> DQHFRGDNEEQEKLLKKSCTLY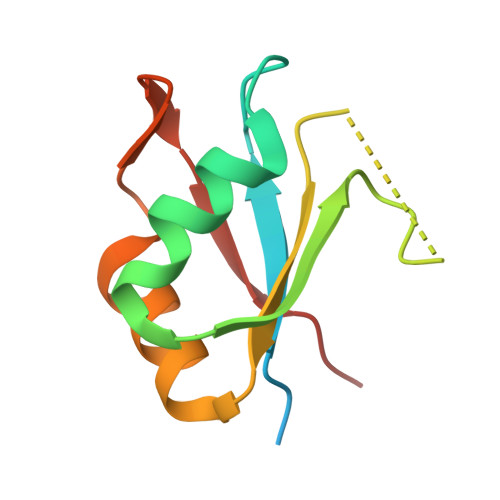VGNLSFYTTEEQIYELFSKSGDIKKIIMGLDKMKTACGFCFVEYYSRADAENAMRYINGTRLDDRIIRTDWDAGFK>AMVRSSSRTPSDKPVAHVVANPQAEGQLQWLNRRANALLANGVELRDNQLVVPSEGLYLIYSQVLFKGQGCPSTHVLLTHTISRIAVSYQTKVNLLSAIKSPCQRETPEGAEA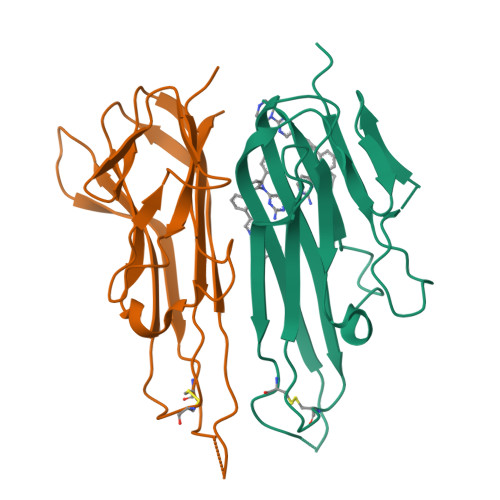KPWYEPIYLGGVFQLEKGDRLSAEINRPDYLDFAESGQVYFGIIAL[48x]>[2x]MDALELLINRRSASRLAEPAPTGEQLQNILRAGMRAPDHKSMQPWHFFVIEGEGRERFSAVLEQGAIAAGSDDKAIDKARNAPFRAPLIITVVAKCEENHKVPRWEQE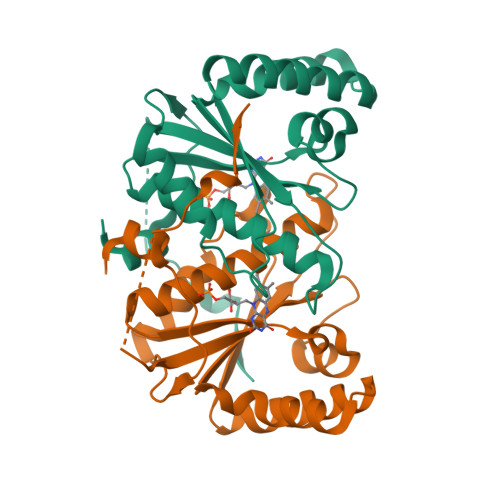MSAGCAVMAMQMAAVAQGFGGIWRSGALTESPVVREAFGCREQDKIVGFLYLGTPQLKASTSINVPDPTPFVTYF>GSHMSDKLPYKVADIGLAAWGRKALDIAENEMPGLMRMRERYSASKPLKGARIAGCLHMTVETAVLIETLVTLGAEVQWSSCNIFSTQDHAAAAIAKAGIPVYAWKGETDEEYLWCIEQTLYFKDGPLNMILDDGGDLTNLIHTKYPQLLPGIRGISEETTTGVHNLYKMMANGILKVPAINVNDSVTKSKFDNLYGCRESLIDGIKRATDVMIAGKVAVVAGYGDVGKGCAQALRGFGARVIITEIDPINALQAAMEGYEVTTMDEACQEGNIFVTTTGCIDIILGRHFEQMKDDAIVCNIGHFDVEIDVKWLNENAVEKVNIKPQVDRYRLKNGRRIILLAEGRLVNLGCAMGHPSFVMS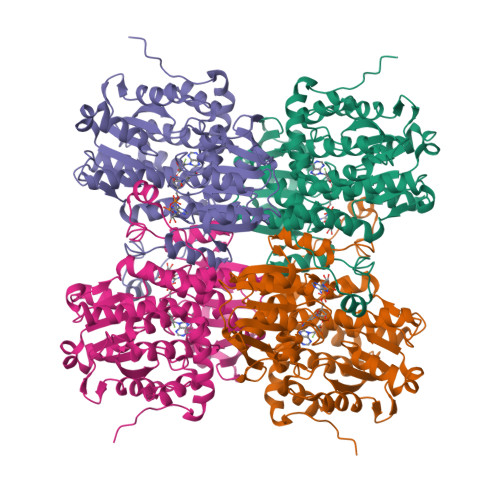NSFTNQVMAQIELWTHPDKYPVGVHFLPKKLDEAVAEAHLGKLNVKLTKLTEKQAQYLGMSCDGPFKPDHYRY[4x]3-HYDROXY-6-METHYL-4-(3-METHYL-2-(3-METHYL-2-(3-METHYL-BUTYRYLAMINO)-BUTYRYLAMINO)-BUTYRYLAMINO)-HEPTANOIC 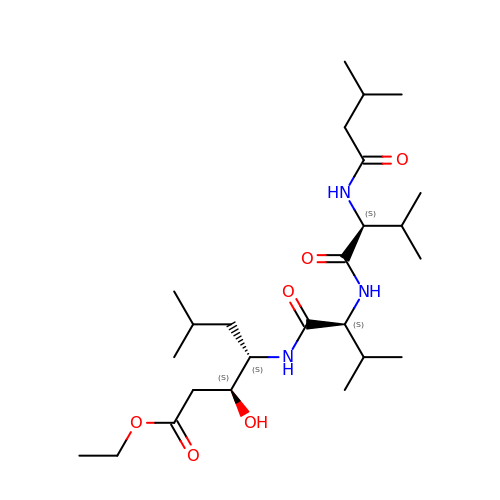ACID ETHYL ESTER | C25 H47 N3 O6 | SMVMSLPPAGGLDL-ZZTDLJEGSA-N> MHLLPLTVSATAVVSAASSPHAKRAAIDECLKNAKVPVTARNSTEWKTDASPFNDRLPYTPAAIAKPATVEHIQAAVLCAAEVGVKANPKSGGHSYASFGLGGEDGHLVVELDRMYNVTLDPETHIATVQPGARLGHIATVLYEEGKRAFSHGTCPGVGVGGHSLHGGFGFSSHSHGLAVDWITSADVVLANGSLVTASETENPDLFWALRGAGSNFGIVASFRFKTFAAPPNVTSYEINLPWTNSSNVVKGWGALQEWLLNGGMPEEMNMRVLGNAFQTQLQGLYHGNASALKTAIQPLLALLDANLSSVQEHDWMEGFRHYAYSGEIDITDPGYDQSETFYSKSLVTSALPPDVLERVAEYWIETANKVRRSWYIIIDMYGGPNSAVTRVPPGAGSYAFRDPERHLFLYELYDRSFGPYPDDGFAFLDGWVHAFTGGLDSSDWGMYINYADPGLDRAEAQEVYYRQNLDRLRRIK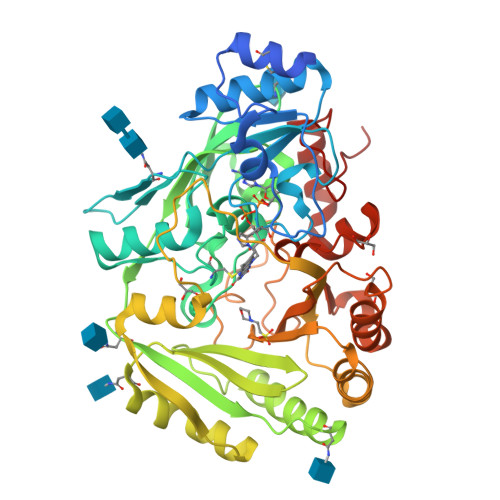QQLDPTELFYYPQAVEPAEV> MALYTPILILGAIAAVFAVVSVGIALVIGPRRFNRSKLEAYECGIDPLPPVAAGLTGQRIPIRYYLIAMLFIVFDIEIVFLYPWAVAFDSLGLFAVIEMLLFMLTVFVAYAYVWRRGGLNWD;> MGLEERLPGGILLSTVETVAGYVRKGSLWPATFGLACCAIEMMSTAGPRFDIARFGMERFSATPRQADLMIVAGRVSQKMAPVLRQIYDQMVEPKWVLAMGVCASSGGMFNNYAVVQGVDHVVPVDIYLPGCPPRPEMLLHAILKLHDKIQQMPLGVNREEAIREAEQAALAVPPTIELKGLLR;> MSTSNGSANGTNGVGLPRGDEPEIIAVRRGMFGNRDTGDTSGYGRLVRPVALPGSTPRPYGGYFDAVMDRLAEVLGEERYAMSIERVVVYRDQLTIEVSRVQLPAVASVLRDDPDLRFELCLGVSGVHYPEDTGRELHAVYPLMSITHNRRIQLEVAAPDADPHIPSLYAVYPTTDWHERETYDFFGIIFDGHPSLTRIEMPDDWEGHPQRKDYPLGGIPVEYHGAQIPPPDQRRSYS;> MSTSTVPPDGGEKVVVVGGNDWHEVVAAARAGAAAQAGERIVVNMGPQHPSTHGVLRLILEIEGEIITEARCGIGYLHTGIEKNLEYRNWTQGVTFVTRMDYLSPFFNETAYCLGVEKLLGITDDIPERASVIRVMLMELNRISSHLVALATGGMELGAMSAMFYGFREREEILRVFESITGLRMNHAYIRPGGLAADLPDDAITQVRRLVEILPKRLKDLEDLLNENYIWKARTVGVGYLDLTGCMALGITGPILRSTGLPHDLRKAQPYCGYENYEFDVITDDRCDSYGRYIIRVKEMHESVKIVEQCLARLKPGPVMISDKKLAWPADLKLGPDGLGNSPEHIAKIMGRSMEGLIHHFKLVTEGIRVPPGQVYVAVESPRGELGVHMVSDGGTRPYRVHYRDPSFTNLQAVAATCEGGMVADAIAAVASIDPVMGGVDR;> MSEVFLELGQRPDEAGPPISGPATYPDDVTESLRADAEQIIARYPDARSALLPLLHLVQAQDGYLTPAGIGFCAAQLGLTEAEVTAVATFYSMYRRTPTGDYLVGVCTNTLCAIMGGDAILEALEDHLGVHPGQTTPDGRVTLEHVECNAACDYAPVVMVNWEFYDNQTPSSARDLVDGLRSGSPPPPTRGSLCTFRETARTLAGLTDPNAPGGAPGAATLAGLRLARERGMTAPTPPQTNGSAS;> MTPLTPVLSRFWDEPEPWTLETYRRHDGYQGLQRALSMGPDDVIAFVKDSGLRGRGGAGFPTGTKWSFIPQERGDQPAGGPAAKPHYLVINADESEPGTCKDIPLLLTTPHFLVEGAIIAAYAIRARHAFIYVRGEVLPVLRRLQAAVAEAYAAGYLGTDIMGSGFDLDLIVHAGAGAYICGEETALLDSLEGRRGQPRLRPPFPAVAGLYACPTVVNNVESIASVPPIMVNGVDWFRSMGSEKSPGFTLYSLSGHVTRPGQYEAPLGITLRELLEYAGGVRAGHQLKFWTPGGSSTPLLTAEHLDVPLDYEGMASVGSMLGTKALQIFDETTCVVRAVRRWTQFYAHESCGKCTPCREGTYWLAQIYARLENGAGTEADIDKLLDISDNIFGKSFCALGDGAASPIMSSIKHFRDEYVAHLDGGCPFDPHASTLMATE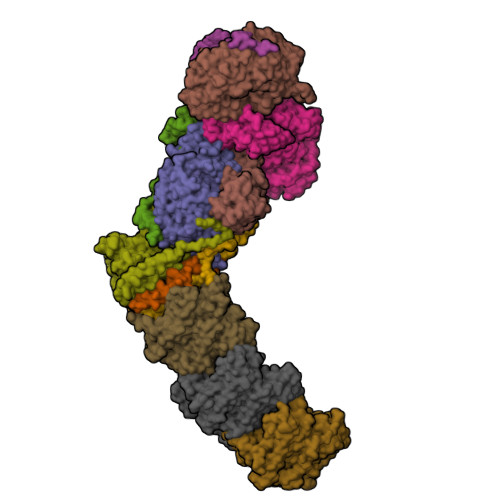GAGV;> MTLAEPTKDTPPVEMVSLTIDDHEISVPKGTLLIRAAELMGIQIPRFCDHPLLDPVGACRQCLVEVEGQRKPMASCTTTVMPDMVVRTQFTSEAADKAQRGVMELLLINHPLDCPICDKGGECPLQNQAMSNGRPETRFEDVKRTFPKPISISSQVLLDRERCVLCARCTRFSSQIAGDPFIDLMERGALQQVGIGQDKPFQSYFSGNTVQICPVGALTGTAYRFRARPFDLVSSPSVCEHCASGCAQRTDHRRGKVLRRLAGDEPEVNEEWNCDKGRWAFTYATVGDRITTPMLRDGGVLRPASWSEALTVAAAGLLTAAGSTGVLVGGRCTVEDAYAYAKFARMVLNTNDVDFRARPHSAEEAEFLAAHVAGQTMGLRYAELENAPTVLLAGFEPEEESPIVFLRLRKGVRKNGVQVVAVAPWASRGLTKLAGTVVPTVPGDEPAALDGMHDDDRLRRPGAVILVGERLATSPGALSAAVRLAAATGARLAWIPRRAGERGAIEAGALPNLLPGGRPVDDADARAEVARAWYISALPEAPGRDTAAILSTAASGHLAALLVGGVELGDLPDPELAVAAVRTTPFVVSLELRESAVTELADVVFPVAPVVEKAGSFLNWEGRPRPFAPSLKTNAIPDLRVLHYLADEIGVDLALPTAEAADAELAQLGTWGGARPPAPTAPPTARPEAGSGQAVLASWRMLLDAGRLQDGEPHLAGTAVRPVARMSAATAAGIGASDGAPVTVSTERGAVTLPLAVTDMPDGVVWLPMNSPGSAVHQRLGVTAGAVVSIGAGA;> MTHPDPTLFGHDPWWLMLAKAVAIFVFLLLTVLSAILIERKLLGRMQMRFGPNRVGPAGLLQSLADGIKLALKEGLVPAGVDKPIYLLAPVISVIPAFVAFSVIPLGGAVSVFGHRTPLQLTDLPVAVLFILAATSIGVYGIVLAGWASGSTYPLLGGLRSSAQVVSYEIAMGLSFVAVFLYAGTMSTSGIVAAQDRTWFVFLLLPSFLVYVVSMVGETNRAPFDLPEAEGELVGGFHTEYSSLKFAMFMLAEYVNMTTVSALATTMFLGGWHAPFPFNLIDGANSGWWPLLWFTAKVWTFMFLYFWLRATLPRLRYDQFMALGWKVLIPVSLLWIMVVAITRSLRQHGEGTWAAWLLTAAVVVVVALIWGLATSLRRRTVQPPPPQSTGAYPVPPLPSVGTKETADA;> MPKFLDALAGFAVTLGSMFKKPITEGYPEKPGPVAPRYHGRHQLNRYPDGLEKCIGCELCAWACPADAIYVEGADNTADERYSPGERYGRVYQINYLRCIGCGLCIEACPTRALTMTTEYEMADDNRADLIWGKDKLLAPLQEGMQAPPHDMAPGKTDDDYYLGNVTPITPVPSGTEDAR;> MNSDLMLLAAEGARTSTSEAVVFWVVGTVALVGAIGVVAARKAVYSAVFLACTMISLAVLYIAQDAPFLGVVQIVVYTGAVMMLFLFVLMLIGVDLTESLVETIKGHRIAALIAGAGFGILVIAGIGNVSVAGFSGLAAANSGGNVEGLAALIFTRYLWAFELTSALLITAALGAMVLAHRERFERRKTQRELAIERFQTGGHPTPLPNPGVYARHNSVDVPARLPDGSESPLSVSTILPHRTVGSATNGKR;> MNPDNYLYLSALLFTIGAAGVLLRRNAIVMFMCVELMLNAANLAFVNFSRMHGQLDGQVVAFFTMVVAACEVVVGLAIIMAIFRTRRSASVDDANLLKH;> MITDWLPVWLLIALPAAGATILLLAGRRSDRWGHLLGCAMSLAAFAVGTVLFAGMLGRSGEERAVHEALFSWVPVGGLQVDFGLQLDQLSVCFVLLITGVGSLIHIYSIGYMAEDPDRRRFFAYLNLFLAAMLLLVLADNYLGLYAGWEGVGLASYLLIGFWSHKPSAATAAKKAFVVNRVGDMGLAIALMIMFATIGSISFAGVFAAAPGLSEATLSAIGLLLLLGACGKSAQVPLQSWLGDAMEGPTPVSALIHAATMVTAGVYLIVRSGPIFDLAPTAQTGVVIVGAVTLLFGAIIGCAKDDIKKALAASTMSQIGYMVLAAGLGPAGYAFAIMHLLTHGFFKAGLFLGAGSVMHAMNDEVNMRRYGGLRKVLPVTFATFGLGYLAIIGVPPLAGFFSKDGIIEAALGAGGARGVILGGAAILGAGITAFYMTRVMLMTFFGEKRWAANSHPHEAPAVMTWPMILLAVGSVVSGGALAIGGTLSHWLEPVVGTHEAHHAVPVWVVTAIVLAVVAVGIAVAYRMYARQAVPEEVPEGSALTVAARRDLYGDAFNEAVFMRGGQTLTAAMVTVDDKAVDGTAGGLAALVSRTSDALRQVQTGFARSYALSMLGGSALVVAAILAVQLW;> MVSTFPWLTVLWAVPVVGAAVVILLPAAQQVLAKWLALAVSVLTLAVTAVVAIGFDPAAAQYQFVESHRWIPSFGTGYILGVDGIALALVVLTAVLVPLLIIAGWNDASRQTGLAGRSVQAYLALTLAVEGMVLMSLVALDILLFYVFFEAMLIPMYFLIGGFGGENRSRAAVKFLLYNLFGGLIMLAAVIGLYVVTAGSDAFAAGTFDFREIVAAVSSGEFAVNPAIMNFLFLGFMFAFAVKAPLWPFHRWLPDAAVEATPASAVLMMAVMDKVGTFGMLRYCLQLFPDASTYFRPVVITLAAIGIVYGAVLAIGQTDVMRLIAYTSISHFGFIILGIFVMTSQGQSGSTLYMINHGISTAALFLIAGFLVSRRGSRLIDSYGGVQKVAPVLAGTFLVAGLATLSLPGLAPFISEFLVLIGTFTRYPVVAVFAATALVLSAVYILWTYQRMMTGPVRDGIGDGDRPVRDLVPRELVVVAPLLALLLVLGIYPKPALDVINPAVEHTLTTIGQTDPEPTVPPTIAEGAR;> MITPSIEYGLLSPMLIVFGVAIAGVLIEALAPRQSRYPLQVTLALGGLIATVVAVVFVARGLSGTPGRPAVLGAVVLDAPAVFLQGTIALVGILGIMLIAERQKATVSAGEARGLEDFTPQASAVAGSVAEQLATKTGVMQTEVFPLTMFAIGGMLLFPAADDLLTMFVALEVLSLPLYLLCGLARRRRLLSQEAALKYFLLGAFSSAFFIYGAAMLYGSAGTLDLSGIAESVAAGSGNTSLALLGVALLLVGVLFKVGAVPFHSWIPDVYQGAPTSITAFMAAATKIAAFGAMLRIFYVAVPALRDDWRPVLWAIAILTMVVGTVTAVTQTDVKRMLAYSAVAHSGFILTGVIAANPAGVSSTLFYLFAYGFSTLGAFAVVGLIRNAAGDEETSMAQWAGLGRRYPIVGVVFSLFLLAFAGIPLTSGFVSKFAVFKAAGEGGAIPLVIIGVIASAVAAYFYVRVIVLMFFTEPPDDAPELVVPSGLSTAVVTVTAAVTFALGALPQPLLDLANSAETFLH;> MAGSAPLRILVYSDNPRTREQVRLALGKRIHPELPEIEYVDVATAPMAISQMDAGGFDLAILDGEATPAGGMGVAKQVKDEIDDCPPILVLTGRADDAWLAKWSRAEAAVPHPIDPIRLSDAVVSLLRAPAQ> DRLGFVVGVVQTGFH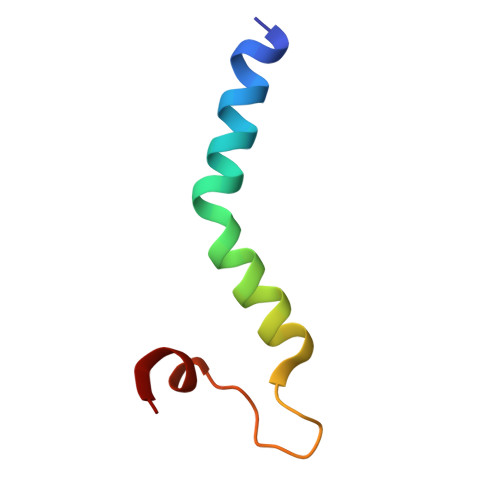WGFVPLVLYLGFMKGAEPGMPPLNLFSLLWQ>MHHHHHHTFGNMERDLFEKKFKEIKDKWVTDKQADEFIETADKYADKAVQMSAVASRAEYYRMYVSRKYQYKKEFVEKLKQVYKESGASHVTSKKDLMLAFDDAKRKSTIGRQENGLFVTSFAEDMALLFTDQGKLKSADQIENIKGVDSGKYSDGVYQYEYDSELTKNIDKLGYIRTASGDTPGANSLNIPGCQTWSGKHIENSESELIFPSISVKDLKSKAVLAEIDAKGYFEIIDPTIIAPNGDHKKVTGRFKIKKMQDRMQDRK[2x];>[2x]MYKVPKGLEHYQKMFQKEVTVNDLKKYLIGSDKEYRIT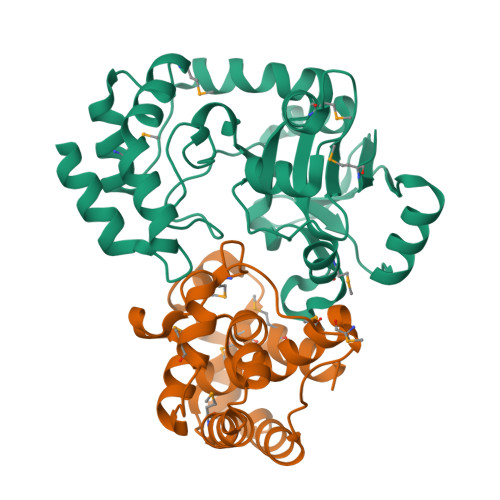RRDSYMGDISDPEVILEYGVYPAFIKGYTQLKANIEEALLEMSNSGQALDIYQAVQTLNAENMLLNYYESLPFYLNRQSILANITKALKDAHIREAMAHYKLGEFAHYQDTMLDMVERTIETF(E)-S-Methyl 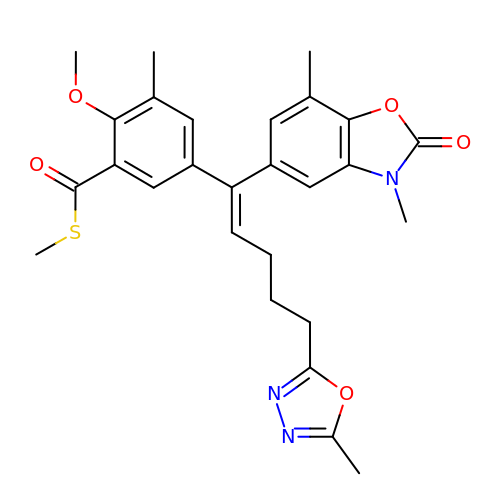5-(1-(3,7-Dimethyl-2-oxo-2,3-dihydrobenzo[d]oxazol-5-yl)-5-(5-methyl-1,3,4-oxadiazol-2-yl)pent-1-enyl)-2-methoxy-3-methylbenzothioate | C27 H29 N3 O5 S | OIXOQSQILWVOGS-AWQFTUOYSA-N>MASAGDVTRAALPRAQPRAEGPACVLGIGTAVPPAEFLQSEYPEFFFNITNCGEKEALKAKFKRICDKSGIRKRHMFLTEEVLKANPGICTYMEPSLNVRHDIVVVQVPKLAAEAAQKAIKEWGGRKSDITHIVFATTSGVNMPGADHALAKLLGLKPTVKRVMMYQTGCFGGASVLRVAKDLAENNKGARVLAVASEVTAVTYRAPSENHLDGLVGSALFGDGAGVYVVGSDPKPEVEKPLFEVHWAGETILPESDGAIDGHLTEAGLIFHL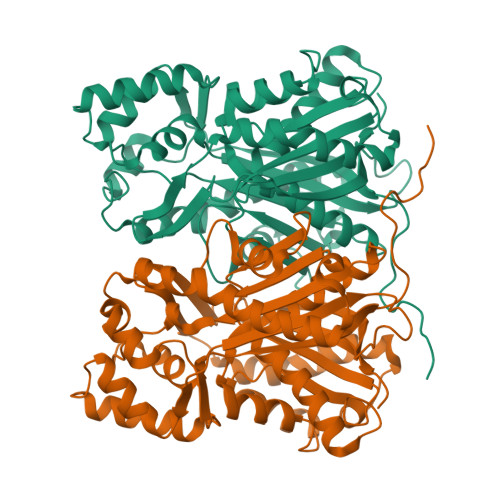MKDVPGLISKNIEKFLNEARKPVGSPAWNEMFWAVHPGGPAILDQVEAKLKLTKDKMQGSRDILSEFGNMSSASVLFVLDQIRHRSVKMGASTLGEGSEFGFFIGFGPGLTLEVLVLRAAPNSA[6x]> SSQIRQNYSTEVEAAVNRLVNLYLRASYTYLSLGFYFDRDDVALEGVCHFFRELAEEKREGAERLLKMQNQRGGRALFQDLQKPS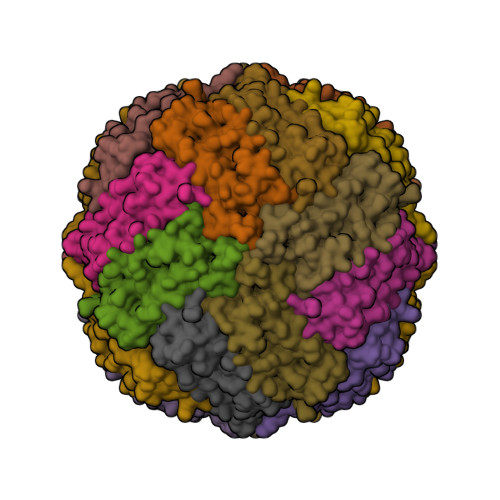QDEWGTTLDAMKAAIVLEKSLNQALLDLHGLGSAQADPHLCDFLESHFLDEEVKLIKKMGDHLTNIQRLVGSQAGLGEYLFERLTLKHD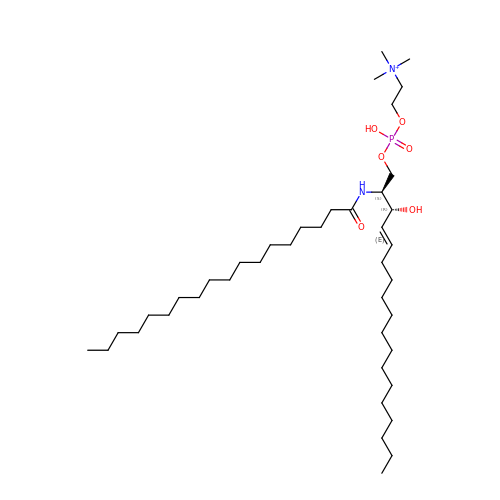Sphingomyelin C18 | C41 H84 N2 O6 P | LKQLRGMMMAHREN-YJFXYUILSA-O>[4x]MKFTLTIAGLLAVGSTAAPTTEKRNPGGIDYVQNYNGDVADFQYNEGAGTYTCGWDGSTDFVVGLGWSTGAARDITYSATYNAGGSGSYLAVYGWVNSP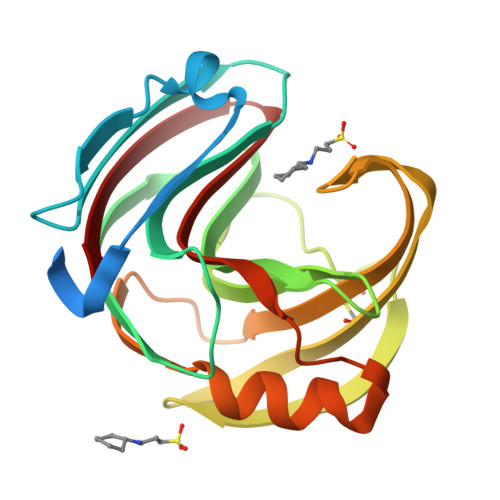QAEYYIVESYGDYNPCSNAEGLGTLESDGSTYTVCTDTRTNEPSITGTSTFTQYWSVRQSERTSGTVTVGNHFNYWAQHGFGDSYNFQVMAVEAFSGSGSASVSVS SPIRAMYCIN I | C43 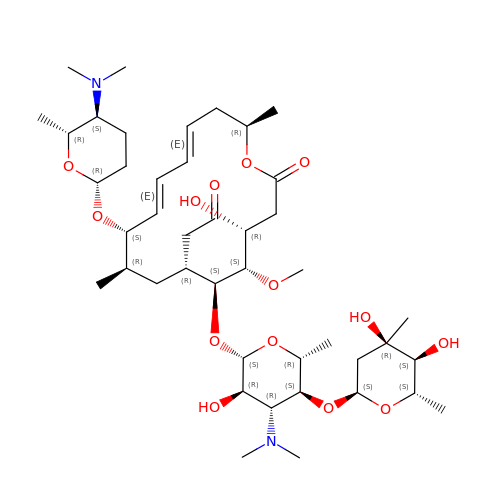H74 N2 O14 | ACTOXUHEUCPTEW-CEUOBAOPSA-N> GSKWKVFIDQINRSLENYEPCSSQNCSCYHGVIEEDLTPFRGGISRKMMAEVVRRKLGTHYQITKNRLYRENDCMFPSRCSGVEHFILEVIGRLPDMEMVINVRDYPQVPKWMEPAIPVFSFSKTSEYHDIMYPAWTFWEGGPAVWPIYPTGLGRWDLFREDLVRSAAQWPWKKKNSTAYFRGSRTSPERDPLILLSRKNPKLVDAEYTKNQAWKSMKDTLGKPAAKDVHLVDHCKYKYLFNFRGVAASFRFKHLFLCGSLVFHVGDEWLEFFYPQLKPWVHYIPVKTDLSNVQELLQFVKANDDVAQEIAERGSQFIRNHLQMDDITCYWENLLSEYSKFLSYNVTRRKGYDQIIP;> GSDGDQCASSPCQNGGSCKDQLQSYICFCLPAFEGRNCETHK

POGLUT1 is an inverting GT-B fold (CAZy GT Family 9018) glycosyltransferase and its EGF-like domain substrates sit in a cleft formed between the canonical N-terminal and C-terminal domains. Here we report the structure of human POGLUT1 in complexes with three different EGF-like domains and either UDP, a donor substrate analog or a slow substrate. The structures reveal the basis for POGLUT1’s ability to recognize diverse EGF-like domain substrates and for the requirement that they be folded. The three EGF-like domains studied are positioned almost identically in their respective complexes and 25–30% of their surface (740–830 Å2) is buried by POGLUT1.

Among the EGF-like domains studied here, EGF(+) (C1ASNPC2) and hEGF12 (C1VSNPC2) do not possess a diserine-containing motif, while hF7EGF1 (C1ASSPC2) does. Of the EGF-like domains studied, hEGF12 and EGF(+) contain an asparagine residue at the Xb position (C1XaSNPC2) while hF7EGF1 contains a serine (C1XaSSPC2). In all cases, the asparagine and serine sidechains make a strong hydrogen bond to the backbone NH group of Gln240. As shown by their UDP complexes, there is little difference between the two EGF-like domain types. In both the POGLUT1/hF7EGF1/UDP and POGLUT1/hEGF12/UDP complexes, the serine hydroxyl is found only in the gauche (−) rotamer where it is hydrogen bonded to the sidechain of the catalytic base and positioned for nucleophilic attack. Moreover, the Xb residue does not make direct or indirect interactions with the donor substrate in either the UDP-CH2-glucose complex or our model for UDP-xylose binding.>[2x]MAEVLVVTSKVKKLIKEKG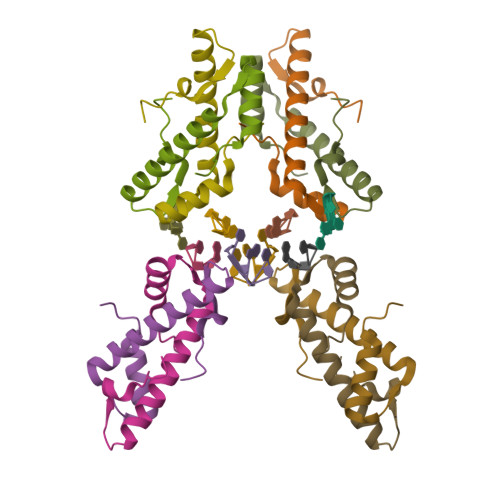QMNTSAETIDVLSKAIEQLCLKGVESAKADGRKTVMARDIVIDHL>MTNKQVEISMAEWDVMNIIWDKKSVSANEIVVEIQKYKEVSDKTIRTLITRLYKKEIIKRYKSENIYFYSSNIKEDDIKMKTAKTFLNKLYGGDMKSLVLNFAKNEELNNKEIEELRDILNDISKK[2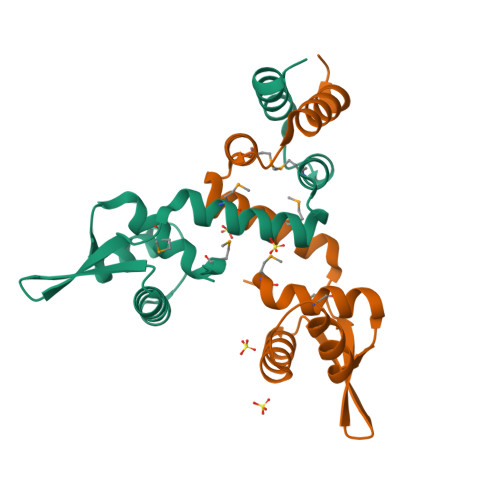x]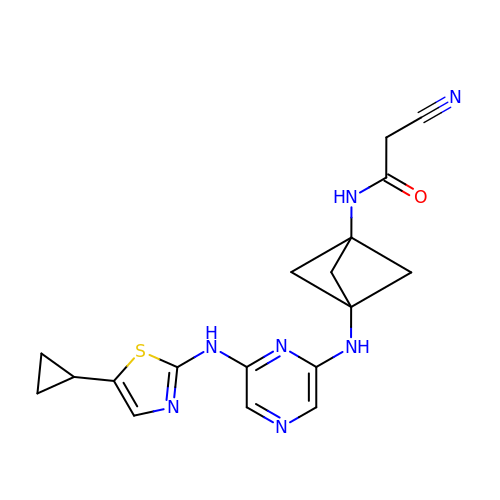2-cyano-N-[3-({6-[(5-cyclopropyl-1,3-thiazol-2-yl)amino]pyrazin-2-yl}amino)bicyclo[1.1.1]pentan-1-yl]acetamide | C18 H19 N7 O S | DYAMAWMMRNCOSW-HDICACEKSA-N> 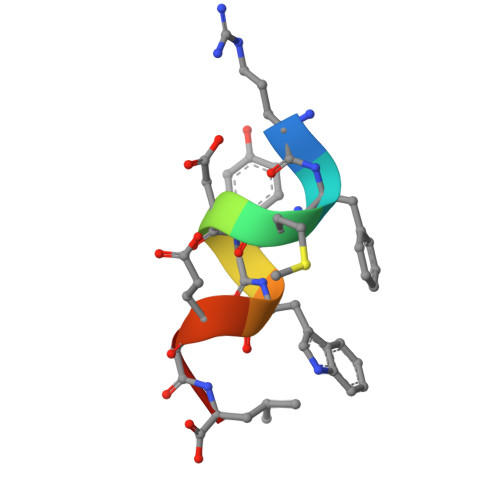RFMDYWEGL N-{cis-4-[(2,6-difluorophenyl)methoxy]cyclohexyl}-N'-(3-phenylpropyl)urea | C23 H28 F2 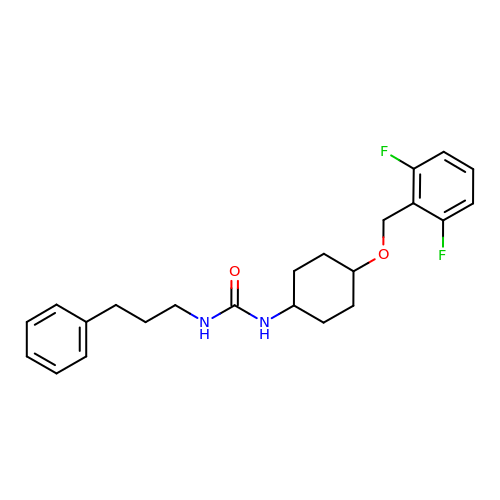N2 O2 | YXIUOVJEXYHABJ-KDURUIRLSA-N>MKIAIAGAGAMGSRFGLMLHQSGNEVLLIDGWAEHVQQIKEHGLQANFNGKEVEAKLPIVLQSEVEKEDQVDLIILFTKAMQLEKMLQDIQSLIKKDTEVLCLLNGIGHEDIIEKFVPMENIYIGNTMWTAGLEGPGQVKLFGSGSVELQNLGDGKEAAAKKLADKLSESGLNAHFSDNIHYSIYRKACVNGTMNGLCTILDVNMAELGKTSTAHKMVATIVNEFAKVAAVEKIELDVPEVIAHCESCFDPETIGLHYPSMYQDLIKNHRLTEIDYINGAISRKGKKYGVATPYCDFLTEL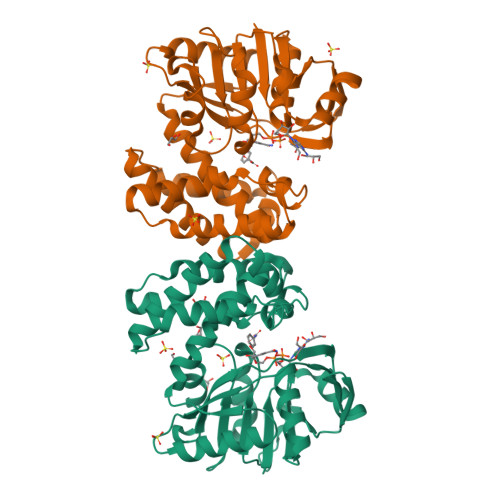VHAKEDSLNVK[6x]>[2x]SNAMKKVQGIYRAPRQHWVGDGFPVRSMFS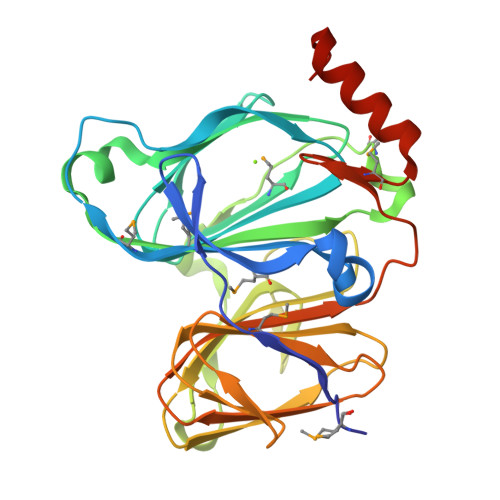YQSHGKQLSPFLLLDYAGPMDFTPTTQRRGVGQHPHRGFETVTIVYHGEVEHRDSTGNGGIIGPGDVQWMTAGAGILHEEFHSDAFAQKGGPFEMVQLWVNLPAKDKMTAPGYQAIRREAIPQVNLPDDAGNLRVIAGEYAGNIGPAKTFSPLNVWDIRLTQGKSCEFSLPAGWNTALIVLHGTLLVNGDAIAREAEMVLLDPTGTHLSIEANNDTVLLLLSGEPIDEPIVGYGPFVMNTQAQIAEAIADFNGGRFGNMDVA>[2x]AMAGVYTYENEFTSDIPAPKLF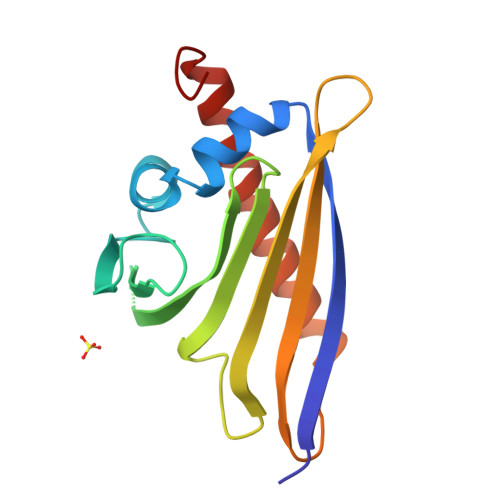KAFVLDADNLIPKIAPQAVKCAEILEGDGGPGTIKKITFGEGSHYGYVKHKIHSIDKVNHTYSYSLIEGDALSENIEKIDYETKLVSAPHGGTIIKTTSKYHTKGDVEIKEEHVKAGKEKAAHLFKLIEGYLKDHPSEYN1-phenyl-2-[(1S,2R,5R,8R,8aR)-1,2,8-trihydroxyoctahydroindolizin-5-yl]ethanone 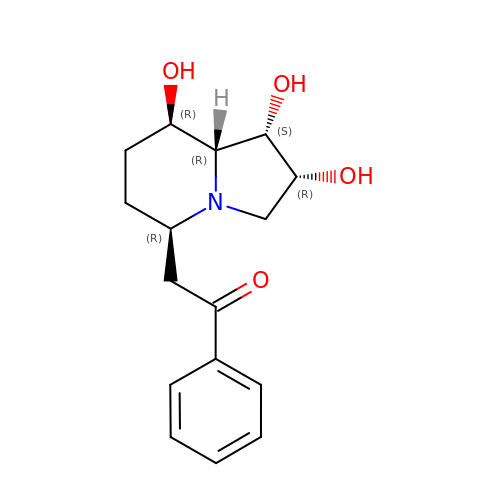| C16 H21 N O4 | HEBIMHSFXQMUTK-CCECPURYSA-N7-chloro-3-{[4-hydroxy-1-(3-phenylpropanoyl)piperidin-4-yl]methyl}quinazolin-4(3H)-one | C23 H24 Cl N3 O3 | 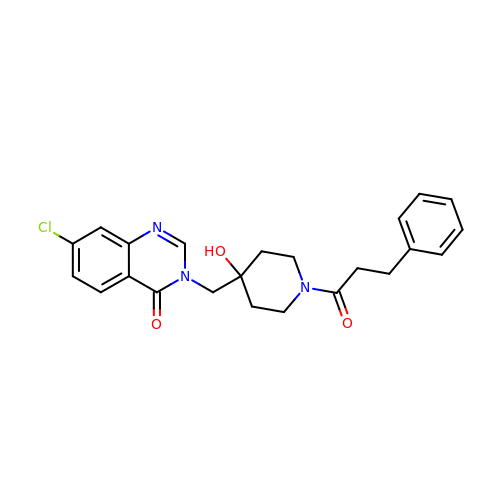CITWIBXKKHFDFM-UHFFFAOYSA-N> SAKALIVYGSTTGNTEYTAETIARELADAGYEVDSRDAASVEAGGLFEGFDLVLLGCSTWGDDSIE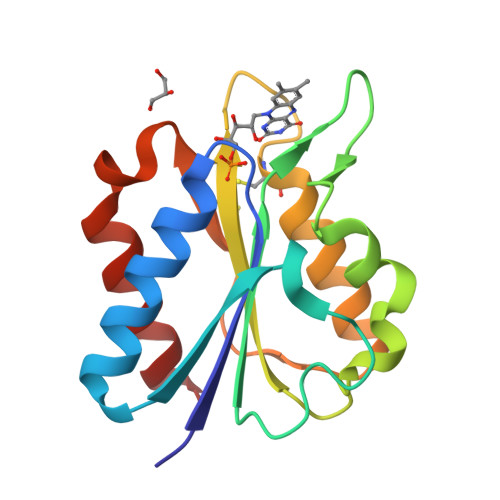LQDDFIPLFDSLEETGAQGRKVACFGCGDSSWEYFCGAVDAIEEKLKNLGAEIVQDGLCIDGDPRAARDDIVGWAHDVRGAI> MRISTQMMYEQNMSGITNSQAEWMKLGEQMSTGKRVTNPSDDPIAASQAVVLSQAQAQNSQYALARTFATQKVSLEESVLSQVTTAIQTAQEKIVYAGNGTLSDDDRASLATDLQGIRDQLMNLANSTDGNGRYIFAGYKTEAAPFDQATGGYHGGEKSVTQQVDSARTMVIGHTGAQIFNSITSNAVPEPDGSDSEKNLFVMLDTAIAALKTPVEGNNVEKEKAAAAIDKTNRGLKNSLNNVLTVRAELGTQLSELSTLDSLGSDRALGQKLQMSNLVDVDWNSVISSYVMQQAALQAS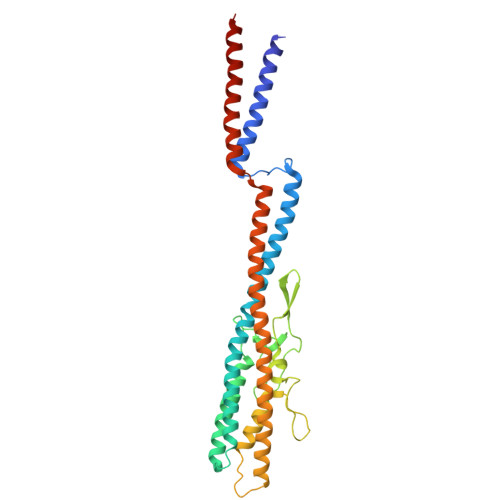YKTFTDMQGMSLFQLNR> MNNKLMNIIELIRKDTGINNAIDAVEQLALLLLVRYTHEVASNEISKENHIDSFKNLFFDLNDFSKDGLVIDFYTLRDKLNHIVVNCRFSENELSHSVFSRNNWEKIENILDQIPFRIRSTKILDLVIHRLEELDLSEGIEIDFDHLLLNMVKDSGSSGAYYSPRPLIKAMVRVLNPKPLATVYDPAMGTGGVFVEAKKHAKGKSCFNGLSFIGNDLSPFAHLIGALNLLLNDIDISGVSISDSLLDRDCQQYDFVISGVPFGKVNELTKYEY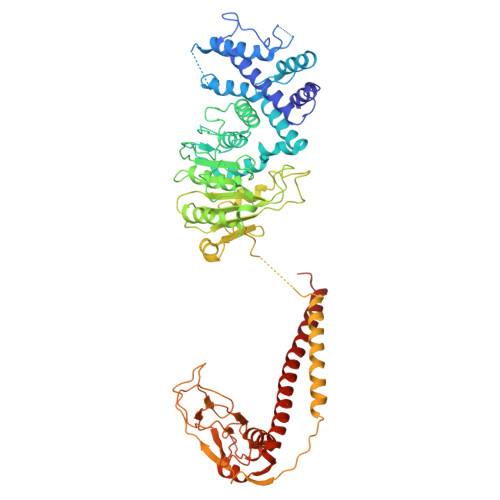YYHGYSGSLEAMFLKHTMDKLAKGGRAAIVIPDGILFGNASHLDELKRQLLTQFNLHAVLSLPKGTLAPYSGVKVSVLFFDNTVSEKDIWFYELRTNKPLSKVNSITDSDFEDFTSLYERREVSENSCLISKESLLQDKTLNLSFSLPKTEAGLKFDKQEMIASLKSEQLSLVTSIENHFDYMSLNLECKYIHQVKLKDICKLRSGDKLNKSEVMDSGEFPVYGGNGVIGFNVEPNRHGDSIVIGKVGAHCGNIHFSTQPYWLTSNAMSLELLDTTKVYLPYLAHVLKSLELNNLATGTAQKFISINKLYEVEVSLPSLEKQREMSEWFTSIEESKSKIQSLLADFSRNLGTISTESITEKALKG> SNAMLGGIEAGGTKFVCAVGREDGTIIDRIEFPTKMPDETIEKVIQYFSQFSLQAIGIGSFGPVDNDKTSQTYGTITATPKAGWRHYPFLQTVKNEMKIPVGFSTDVNAAALGEFLFGEAKGLDSCLYITIGTGIGAGAIVEGRLLQGLSHPEMGHIYIRRHPDDVYQGKCPYHGDCFEGLASGPAIEARWGKKAADLSDIAQVWELEGYYIAQALAQYILILAPKKIILGGGVMQQKQVFSYIYQYVPKIMNSYLDFSELSDDISDYIVPPRLGSNAGIIGTLVLA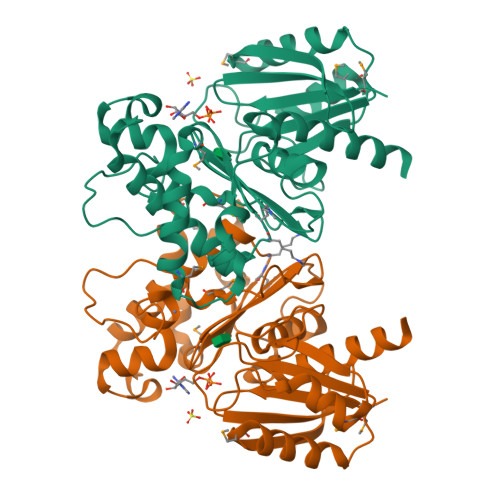HQALQAEAASGEVRS Uniquely, the sulfonylurea receptors SUR1 and SUR2 lack transport activity per se but instead are devoted to forming the ATP-sensitive potassium (KATP) channels, wherein four SUR.x subunits form a complex with four subunits of an inwardly rectifying potassium channel, Kir6.1 or Kir6.2. KATP channels are gated by intracellular ATP and ADP, key features which enable them to regulate membrane excitability according to the energetic state of the cell. In pancreatic β-cells, KATP channels composed of SUR1 and Kir6.2 couple glucose metabolism to insulin secretion. The SUR1 protein has an N-terminal transmembrane domain referred to as TMD0 that interacts directly with the Kir6.2 subunit, followed by a cytoplasmic loop termed L0, and then the ABC core structure comprising two transmembrane domains TMD1 and TMD2 and two nucleotide binding domains NBD1 and NBD2.

Here, in both the RPG/ATP and CBZ/ATP structures, we observe strong and distinctly shaped cryo-EM densities within the same GBC binding pocket. Density for RPG appears compact and palm-shaped, and suggests that the molecule adopts a considerably folded shape upon binding to SUR1. Interestingly, RPG possesses a carboxyl group adjacent a benzyl group, analogous to the sulfonyl group in GBC that is also adjacent a benzyl group. Refinement of an RPG molecule into the observed binding pocket density orients this carboxylate towards N1245, R1246, and R1300, which coordinate the sulfonyl group in the GBC-bound structure. However, unlike GBC, the RPG density is distant from S1238. This explains previous functional data that an SUR1 S1238Y mutation does not affect RPG’s ability to modulate channel function. Interestingly, although similar in overall structures, we noted subtle rearrangements within the binding pocket between GBC- and RPG-bound states. The most obvious is in W1297, which in RPG is flipped down towards the ligand. Interestingly, in the RPG-bound structure the piperidino moiety of RPG is in close proximity to the density that corresponds to the most N-terminus of the KNt. This observation agrees with previous findings that the increased affinity to RPG caused by Kir6.2 is due to the peperidino group, and that deletion of only a few amino acids from the Kir6.2 N-terminus decreases RPG binding affinity by more than 30-fold.

> MPLAFCGTENHSAAYRVDQGVLNNGCFVDALNVVPHVFLLFITFPILFIGWGSQSSKVHIHHSTWLHFPGHNLRWILTFILLFVLVCEIAEGILSDGVTESRHLHLYMPAGMAFMAAITSVVYYHNIETSNFPKLLIALLIYWTLAFITKTIKFVKFYDHAIGFSQLRFCLTGLLVILYGMLLLVEVNVIRVRRYIFFKTPREVKPPEDLQDLGVRFLQPFVNLLSKGTYWWMNAFIKTAHKKPIDLRAIAKLPIAMRALTNYQRLCVAFDAQARKDTQSPQGARAIWRALCHAFGRRLILSSTFRILADLLGFAGPLCIFGIVDHLGKENHVFQPKTQFLGVYFVSSQEFLGNAYVLAVLLFLALLLQRTFLQASYYVAIETGINLRGAIQTKIYNKIMHMSTSNLSMGEMTAGQICNLVAIDTNQLMWFFFLCPNLWTMPVQIIVGVILLYYILGVSALIGAAVIILLAPVQYFVATKLSQAQRTTLEHSNERLKQTNEMLRGMKLLKLYAWESIFCSRVEVTRRKEMTSLRAFAVYTSISIFMNTAIPIAAVLITFVGHVSFFKESDLSPSVAFASLSLFHILVTPLFLLSSVVRSTVKALVSVQKLSEFLSSAEIREEQCAPREPAPQGQAGKYQAVPLKVVNRKRPAREEVRDLLGPLQRLAPSMDGDADNFCVQIIGGFFTWTPDGIPTLSNITIRIPRGQLTMIVGQVGCGKSSLLLATLGEMQKVSGAVFWNSNLPDSEGEDPSSPERETAAGSDIRSRGPVAYASQKPWLLNATVEENITFESPFNKQRYKMVIEACSLQPDIDILPHGDQTQIGERGINLSGGQRQRISVARALYQQTNVVFLDDPFSALDVHLSDHLMQAGILELLRDDKRTVVLVTHKLQYLPHADWIIAMKDGTIQREGTLKDFQRSECQLFEHWKTLMNRQDQELEKETVMERKASEPSQGLPRAMSSRDGLLLDEEEEEEEAAESEEDDNLSSVLHQRAKIPWRACTKYLSSAGILLLSLLVFSQLLKHMVLVAIDYWLAKWTDSALVLSPAARNCSLSQECDLDQSVYAMVFTLLCSLGIVLCLVTSVTVEWTGLKVAKRLHRSLLNRIILAPMRFFETTPLGSILNRFSSDCNTIDQHIPSTLECLSRSTLLCVSALTVISYVTPVFLVALLPLAVVCYFIQKYFRVASRDLQQLDDTTQLPLVSHFAETVEGLTTIRAFRYEARFQQKLLEYTDSNNIASLFLTAANRWLEVCMEYIGACVVLIAAATSISNSLHRELSAGLVGLGLTYALMVSNYLNWMVRNLADMEIQLGAVKRIHALLKTEAESYEGLLAPSLIPKNWPDQGKIQIQNLSVRYDSSLKPVLKHVNTLISPGQKIGICGRTGSGKSSFSLAFFRMVDMFEGRIIIDGIDIAKLPLHTLRSRLSIILQDPVLFSGTIRFNLDPEKKCSDSTLWEALEIAQLKLVVKALPGGLDAIITEGGENFSQGQRQLFCLARAFVRKTSIFIMDEATASIDMATENILQKVVMTAFADRTVVTIAHRVHTILSADLVMVLKRGAILEFDKPETLLSQKDSVFASFVRADK;> MLSRKGIIPEEYVLTRLAEDPTEPRYRTRERRARFVSKKGNCNVAHKNIREQGRFLQDVFTTLVDLKWPHTLLIFTMSFLCSWLLFAMVWWLIAFAHGDLAPGEGTNVPCVTSIHSFSSAFLFSIEVQVTIGFGGRMVTEECPLAILILIVQNIVGLMINAIMLGCIFMKTAQAHRRAETLIFSKHAVITPRHGRLCFMLRVGDLRKSMIISATIHMQVVRKTTSPEGEVVPLHQVDIPMENGVGGNSIFLVAPLIIYHVIDSNSPLYDLAPSDLHHHQDLEIIVILEGVVETTGITTQARTSYLADEILWGQRFVPIVAEEDGRYSVDYSKFGNTVKVPTPLCTARQLDEDRSLLDALTLASSRGPLRKRSVAVAKAKPKFSISPDSLS>[2x]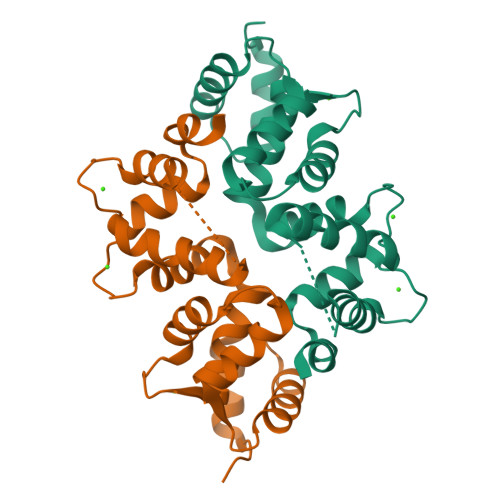MGKKNSKLKQDTIDRLTTDTYFTEKEIRQWHKGFLKDCPNGLLTEQGFIKIYKQFFPDGDPSKFASLVFRVFDENNDGAIEFEEFIRALSITSRGNLDEKLHWAFRLYDVDNDGYITREEMYNIVDAIYQMVGQQPQTEDENTPQKRVDKIFDQMDKNHDDRLTLEEFREGSKADPRMVQALSLGGD>MHHHHHHAAGIPMNNPAIKRIGNHITKSPEDKRE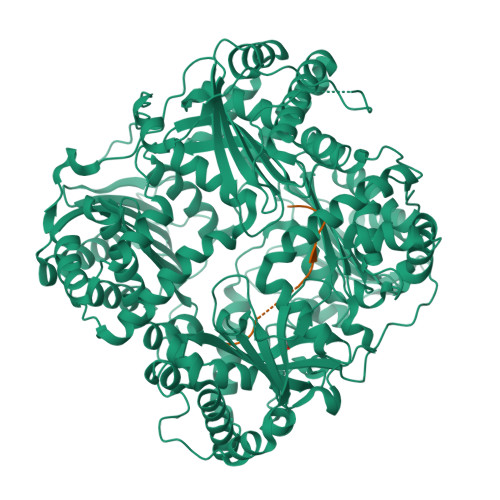YRGLELANGIKVLLISDPTTDKSSAALDVHIGSLSDPPNIAGLSHFCQHMLFLGTKKYPKENEYSQFLSEHAGSSNAFTSGEHTNYYFDVSHEHLEGALDRFAQFFLCPLFDESCKDREVNAVDSEHEKNVMNDAWRLFQLEKATGNPKHPFSKFGTGNKYTLETRPNQEGIDVRQELLKFHSAYYSSNLMAVCVLGRESLDDLTNLVVKLFSEVENKNVPLPEFPEHPFQEEHLKQLYKIVPIKDIRNLYVTFPIPDLQKYYKSNPGHYLGHLIGHEGPGSLLSELKSKGWVNTLVGGQKEGARGFMFFIINVDLTEEGLLHVEDIILHMFQYIQKLRAEGPQEWVFQECKDLNAVAFRFKDKERPRGYTSKIAGILHYYPLEEVLTAEYLLEEFRPDLIEMVLDKLRPENVRVAIVSKSFEGKTDRTEEWYGTQYKQEAIPDEVIKKWQNADLNGKFKLPTKNEFIPTNFEILPLEKEATPYPALIKDTAMSKLWFKQDDKFFLPKACLNFEFFSPFAYVDPLHCNMAYLYLELLKDSLNEYAYAAELAGLSYDLQNTIYGMYLSVKGYNDKQPILLKKIIEKMATFEIDEKRFEIIKEAYMRSLNNFRAEQPHQHAMYYLRLLMTEVAWTKDELKEALDDVTLPRLKAFIPQLLSRLHIEALLHGNITKQAALGIMQMVEDTLIEHAHTKPLLPSQLVRYREVQLPDRGWFVYQQRNEVHNNCGIEIYYQTDMQSTSENMFLELFCQIISEPCFNTLRTKEQLGYIVFSGPRRANGIQGLRFIIQSEKPPHYLESRVEAFLITMEKSIEDMTEEAFQKHIQALAIRRLDKPKKLSAECAKYWGEIISQQYNFDRDNTEVAYLKTLTKEDIIKFYKEMLAVDAPRRHKVSVHVLAREMDSCPVVGEFPCQNDINLSQAPALPQPEVIQNMTEFKRGLPLFPLVKPHINFMAAKL[2x];>HSQGTFTSDYSKYLDSRRAQDFVQWLMNT[2x]>[6x]MQILWKKYVKENFEMNVDECGIEQGIPGLGYNYEVLKNAVIHYVTKGYGTFKFNGKVYNLKQGDIFILLKGMQVEYVASIDDPWEYYWIGFSG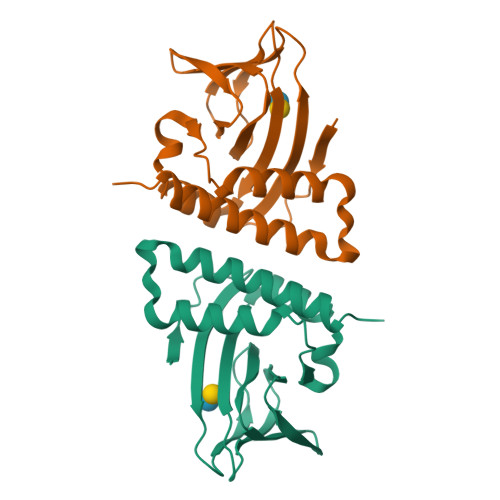SNANEYLNRTSITNSCVANCEENSKIPQIILNMCEISKTYNPSRSDDILLLKELYSLLYALIEEFPKPFEYKDKELHLVPRGSHHHHHH> MSEESQAFQRQLTALIGYDVTDVSNVHDDELEFTRRGLVTPRMAEVASRDPKLYAMHPWVTSKPLPEYLWKKIANNCIFIVIHRSTTSQTIKVSPDDTPGAILQSFFTKMAKKKSLMDIPESQSEQDFVLRVCGRDEYLVGETPIKNFQWVRHCLKNGEEIHVVLDTPPDPALDEVRKEEWPLVDDCTGVTGYHEQLTIHGKDHESVFTVSLWDCDRKFRVKIRGIDIPVLPRNTDLTVFVEANIQHGQQVLCQRRTSPKPFTEEVLWNVWLEFSIKIKDLPKGALLNLQIYCGKAPALSSKASAESPSSESKGKVQLLYYVNLLLIDHRFLLRRGEYVLHMWQISGKGEDQGSFNADKLTSATNPDKENSMSISILLDNYCHPIALPKHQPTPDPEGDRVRAEMPNQLRKQLEAIIATDPLNPLTAEDKELLWHFRYESLKHPKAYPKLFSSVKWGQQEIVAKTYQLLARREVWDQSALDVGLTMQLLDCNFSDENVRAIAVQKLESLEDDDVLHYLLQLVQAVKFEPYHDSALARFLLKRGLRNKRIGHFLFWFLRSEIAQSRHYQQRFAVILEAYLRGCGTAMLHDFTQQVQV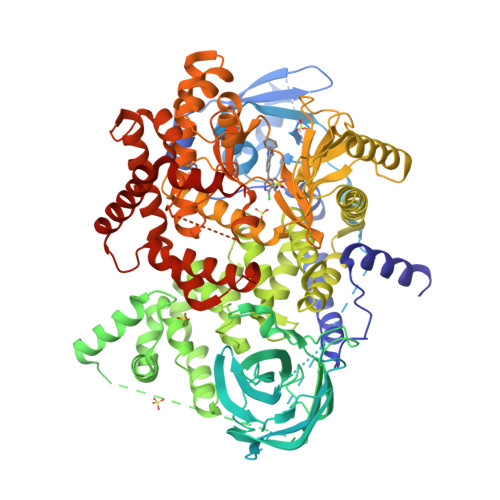IEMLQKVTLDIKSLSAEKYDVSSQVISQLKQKLENLQNSQLPESFRVPYDPGLKAGALAIEKCKVMASKKKPLWLEFKCADPTALSNETIGIIFKHGDDLRQDMLILQILRIMESIWETESLDLCLLPYGCISTGDKIGMIEIVKDATTIAKIQQSTVGNTGAFKDEVLNHWLKEKSPTEEKFQAAVERFVYSCAGYCVATFVLGIGDRHNDNIMITETGNLFHIDFGHILGNYKSFLGINKERVPFVLTPDFLFVMGTSGKKTSPHFQKFQDICVKAYLALRHHTNLLIILFSMMLMTGMPQLTSKEDIEYIRDALTVGKNEEDAKKYFLDQIEVCRDKGWTVQFNWFLHLVLGIKQGEKHSAHHHHHH(1R,5S)-7-{4-[3-(2-chloro-3,6-difluorophenoxy)propyl]phenyl}-N-cyclopropyl-N-(2,3-dichlorobenzyl)-3,9-diazabicyclo[3.3.1]non-6-ene-6-carboxamide | C33 H32 Cl3 F2 N3 O2 | 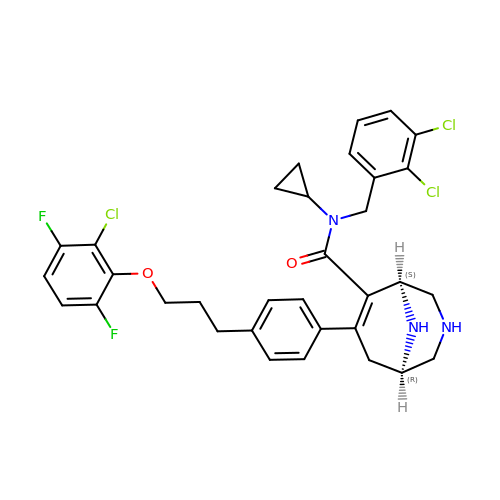SXZFQYPWEANJGQ-SKCUWOTOSA-N> MDINIDDILAELDKETTAVDSTKITQGSSSTTHRDANTIVGSSLDLNDKTQIYVSPQQDFSDLMKSWKNERCSPELLPYPHQLMKRLLNRISMQSQLIENISMGFLDMQNASNANPPMPNESKLPLLCMETELERLKFVIRSYIRCRL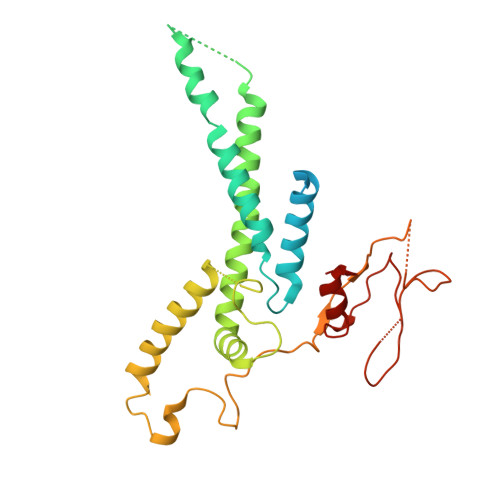SKIDKFSLYLRQLNEDENSLISLTDLLSKDEIKYHDTHSLIWLKLVNDSILKYMPEELQAINDTEGSVNMIDEPDWNKFVFIHVNGPPDGKWNEDPLLQENEFGKPCYTVTIPDLKEEVELTIGSIYVMRYEVIRDLLRDDKVALI>[2x]MARKYFVAANWKCNGTLESIKSLTNSFNNLDFDPSKLDVVVFPVSVHYDHTRKLLQSKFSTGIQNVSKFGNGSYTGEVSAEIAKDLNIEYVIIGHWERRKY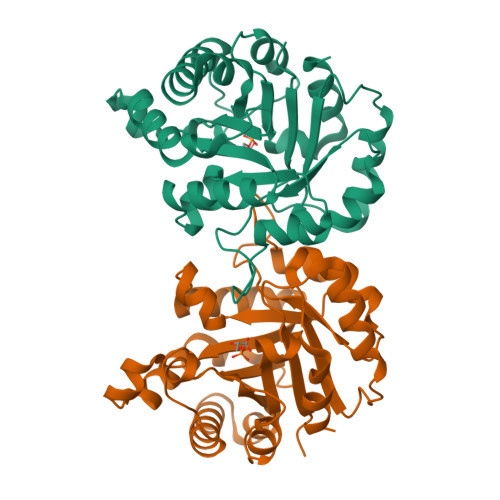FHETDEDVREKLQASLKNNLKAVVCFGESLEQREQNKTIEVITKQVKAFVDLIDNFDNVILVYEPLWAIGTGKTATPEQAQLVHKEIRKIVKDTCGEKQANQIRILYGGSVNTENCSSLIQQEDIDGFLVGNASLKESFVDIIKSAM> SDFYLPGDYLLGGLFSLHANMKGIVHLNFLQVPMCKEYEVKVIGYNLMQAMRFAVEEINNDSSLLPGVLLGYEIVDVCYISNNVQPVLYFLAHEDNLLPIQEDYSNYSSRVVAVIGPDNSESVMTVANFLSLFLLPQITYSAISDELRDKVRFPALLRTTPSADHHIEAMVQLMLHFRWNWIIVLVSNDTYGRDNGQLLGERVARRGICIAFQETLPTLQPNQNMTSEERQRLVTIVDKLQQSTARVVVVFSPDLTLYHFFNEVLRQNFTGAVWIASESWAIDPVLHNLTELRHLGTFLGITIQSVPIPGFSEFREWGPQAGPPPLSRTSQSYTCNQECDNCLNATLSFNTILRLSGERVVYSVY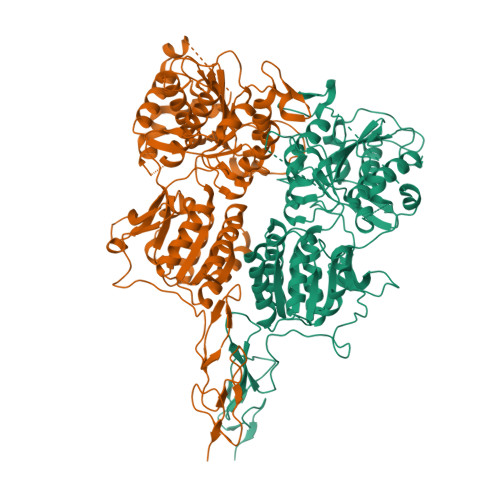SAVYAVAHALHSLLGCDKSTCTKRVVYPWQLLEEIWKVNFTLLDHQIFFDPQGDVALHLEIVQWQWDRSQNPFQSVASYYPLQRQLKNIQDISWHTINNTIPMSMCSKRCQSGQKKKPVGIHVCCFECIDCLPGTFLNHTEDEYECQACPNNEWSYQSETSCFKRQ;> LCLSQQFKAQGDYILGGLFPLGSTEEATLNQRTQPNSIPCNRFSPLGLFLAMAMKMAVEEINNGSALLPGLRLGYDLFDTCSEPVVTMKSSLMFLAKVGSQSIAAYCNYTQYQPRVLAVIGPHSSELALITGKFFSFFLMPQVSYSASMDRLSDRETFPSFFRTVPSDRVQLQAVVTLLQNFSWNWVAALGSDDDYGREGLSIFSSLANARGICIAHEGLVPQHDTSGQQLGKVLDVLRQVNQSKVQVVVLFASARAVYSLFSYSIHHGLSPKVWVASESWLTSDLVMTLPNIARVGTVLGFLQRGALLPEFSHYVETHLALAADPAFCASLNAELDLEEHVMGQRCPRCDDIMLQNLSSGLLQNLSAGQLHHQIFATYAAVYSVAQALHNTLQCNVSHCHVSEHVLPWQLLENMYNMSFHARDLTLQFDAEGNVDMEYDLKMWVWQSPTPVLHTVGTFNGTLQLQQSKMYWPGNQVPVSQCSRQCKDGQVRRVKGFHSCCYDCVDCKAGSYRKHPDDFTCTPCNQDQWSPEKSTACLPRR ethyl 2-oxopropanoate 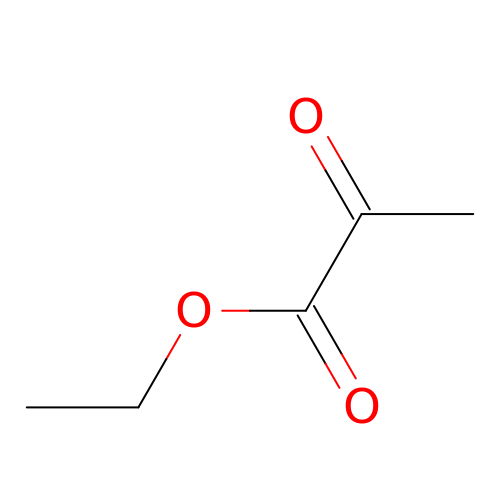| C5 H8 O3 | XXRCUYVCPSWGCC-UHFFFAOYSA-N>MNMDVIKSFTEQMQGFAAPLTRYNQLLASNIEQLTRLQLASANAYAELGLNQLQAVSKVQDTQSLAALGTVQLETASQLSRQMLD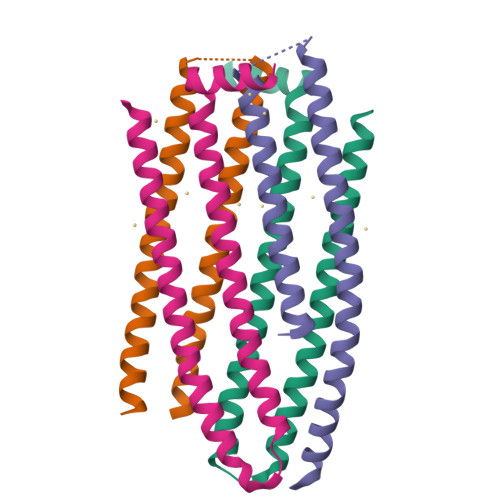DIQKLSALGQQFKEELDVLTADGIKKSTGKA[16x]>GQTWEPLFNGKNLKGWKKLNGKAEYKIVDGAIVGISKMGTPNTFLATTKNYGDFILEFDFKIDDGLNSGVQLRSESKKDYQNGRVHGYQFEIDPSKRAWSGGIYDEARRNWLYPLTLNPAAKTAFKNNAWNKARIEAIGNSIRTWINGVPCANIWDDMTPSGFIALQVHAIGNASEEGKTVSWKDIRICTTDVERYQTPETEEAPERNMIANTISPREAKEGWALLWDGKTNNGWRGAKLNAFPEKGWKMEDGILKVMKSGGAESANGGDIVTTRKYKNFILTVDFKITEGANSGVKYFVNPDLNKGEGSAIGCEFQILDDDKHPDAKLGVKGNRKLGSLYDLIPAPEKKPFNKKDFNTATIIVQDNHVEHWLNGVKLIEYTRNTDMWNALVAYSK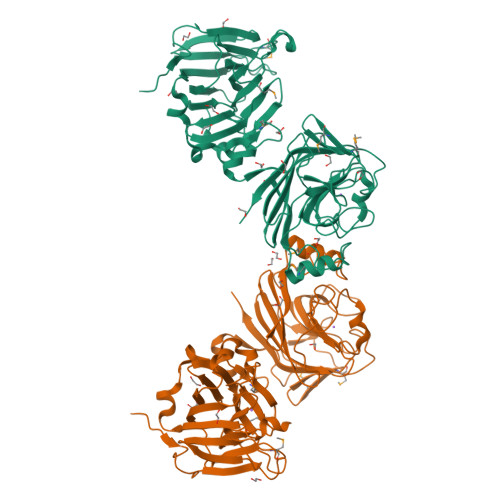YKNWPNFGNSAEGNILLQDHGDEVWFKNVKIKELK[2x]> MSMLKREDWYDLTRTTNWTPKYVTENELFPEEMSGARGISMEAWEKYDEPYKITYPEYVSIQREKDSGAYSIKAALERDGFVDRADPGWVSTMQLHFGAIALEEYAASTAEARMARFAKAPGNRNMATFGMMDENRHGQIQLYFPYANVKRSRKWDWAHKAIHTNEWAAIAARSFFDDMMMTRDSVAVSIMLTFAFETGFTNMQFLGLAADAAEAGDHTFASLISSIQTDESRHAQQGGPSLKILVENGKKDEAQQMVDVAIWRSWKLFSVLTGPIMDYYTPLESRNQSFKEFMLEWIVAQFERQLLDLGLDKPWYWDQFMQDLDETHHGMHLGVWYWRPTVWWDPAAGVSPEEREWLEE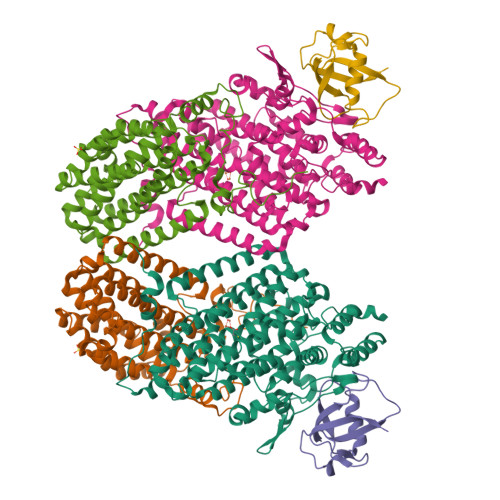KYPGWNDTWGQCWDVITDNLVNGKPELTVPETLPTICNMCNLPIAHTPGNKWNVKDYQLEYEGRLYHFGSEADRWCFQIDPERYKNHTNLVDRFLKGEIQPADLAGALMYMSLEPGVMGDDAHDYEWVKAYQKKTNAA;> MSEQQPEALKPLKTWSHLAGNRRRPSEYEVVSTNLHYFTDNPERPWELDSNLPMQTWYKKYCFDSPLKHDDWNAFRDPDQLVYRTYNLLQDGQESYVQGLFDQLNDRGHDQMLTREWVETLARFYTPARYLFHALQMGSVYIHQIAPASTITNCATYETADHLRWLTHTAYRTRELANCYPDVGFGKRERDVWENDPAWQGFRELIEKALIAWDWGEAFTAINLVTKPAVEEALLQQLGSLAQSEGDTLLGLLAQAQKRDAERHRRWSSALVKMALEKEGNREVLQKWVAKWEPLADKAIEAYCSALPDGENAIVEAKSASRYVRQMMGL;> MATFPIMSNFERDFVIQLVPVDTEDTMDQVAEKCAYHSINRRVHPQPEKILRVRRHEDGTLFPRGMIVSDAGLRPTETLDIIFMDN> RERPHTSGHHGAGEARATAPSTVSPYGPEARAELSSRLTTLRNTLAPATNDPRY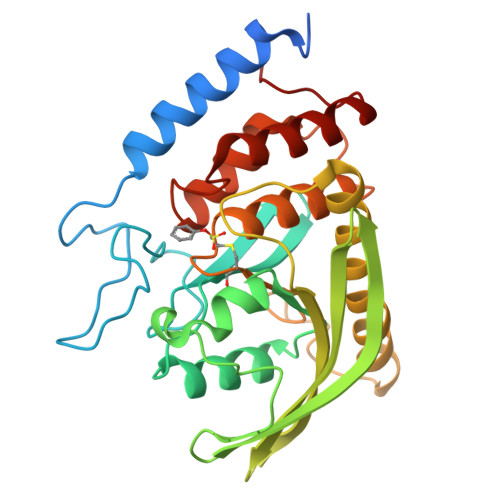LQACGGEKLNRFRDIQCRRQTAVRADLNANYIQVGNTRTIACQYPLQSQLESHFRMLAENRTPVLAVLASSSEIANQRFGMPDYFRQSGTYGSITVESKMTQQVGLGDGIMADMYTLTIREAGQKTISVPVVHVGNWPAQTAVSSEVTKALASLVDQTAETKRNMYESKGSSAVADDSKLRPVIHCRAGVGRTAQLIGAMCMNDSRNSQLSVEDMVSQMRVQRNGIMVQKDEQLDVLIKLAEGQGRPLLNS> GGGTMQVQCQQSPVLAGSATLVALGALALYVAKPSGYGKHTESLKPAATRLPARAAWFLQELPSFAVPAGILARQPLSLFGPPGTVLLGLFCVHYFHRTFVYSLLNRGRPYPAILILRGTAFCTGNGVLQGYYLIYCAEYPDGWYTDIRFSLGVFLFILGMGINIHSDYILRQLRKPGEISYRIPQGGLFTYVSGANFLGEIIEWIGYALATWSL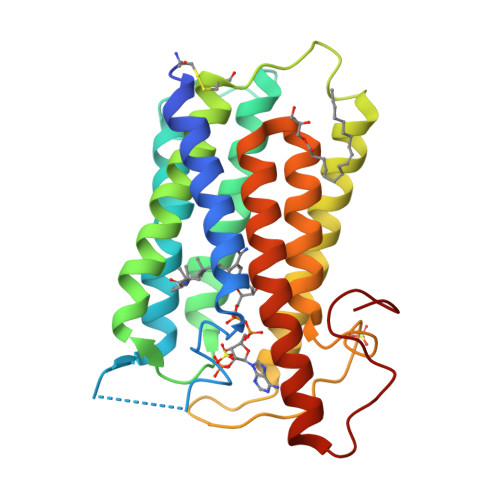PALAFAFFSLCFLGLRAFHHHRFYLKMFEDYPKSRKALIPFIF>[2x]NTIQQLMMILNSASDQPSENLISYFNNCTVNPKESILKRVKDIGYIFKEKFAKAVGQGCVEIGSQRYKLGVRLYYRVMESMLKSEEERLSIQNFSKLLNDNIFHMSLLACALEVVMATYSRSTSQNLDS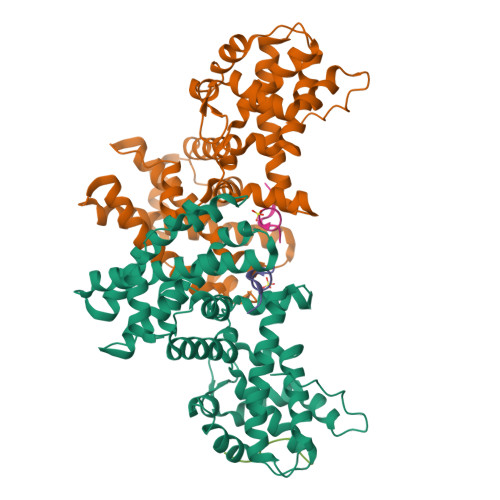GTDLSFPWILNVLNLKAFDFYKVIESFIKAEGNLTREMIKHLERCEHRIMESLAWLSDSPLFDLIKQSKDREGKSTSLSLFYKKVYRLAYLRLNTLCERLLSEHPELEHIIWTLFQHTLQNEYELMRDRHLDQIMMCSMYGICKVKNIDLKFKIIVTAYKDLPHAVQETFKRVLIKEEEYDSIIVFYNSVFMQRLKTNILQYASTRPPTLSPIPHIPR;>[3x]PPTLHELYDL> MDSYSAPESTPSASSRPEDYFIGATPLQKRLESVRKQSSFILTPPRRKIPQCSQLQEDVDPQKVAFLLHKQWTLYSLTPLYKFSYSNLKEYSRLLNAFIVAEKQKGLAVEVGEDFNIKVIFSTLLGMKGTQRDPEAFLVQIVSKSQLPSENREGKVLWTGWFCCVFGDSLLETVSEDFTCLPLFLANGAESNTAIIGTWFQKTFDCYFSPLAINAFNLSWMAAMWTACKMDHYVATTEFLWSVPCSPQSLDISFAIHPEDAKALWDSVHKTPGEVT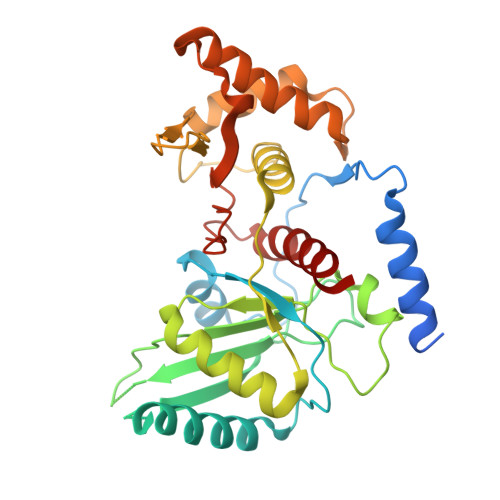QEEVDLFMDCLYSHFHRHFKIHLSATRLVRVSTSVASAHTDGKIKILCHKYLIGVLAYLTELAIFQIE> HPKLVSSTPAEGSEGAAPAKIELHFSENLVTQFSGAKLVMTAMPGMEHSPMAVKAAVSGGGDPKTMVITPASPLTAGTYKVDWRAVSSDTFPI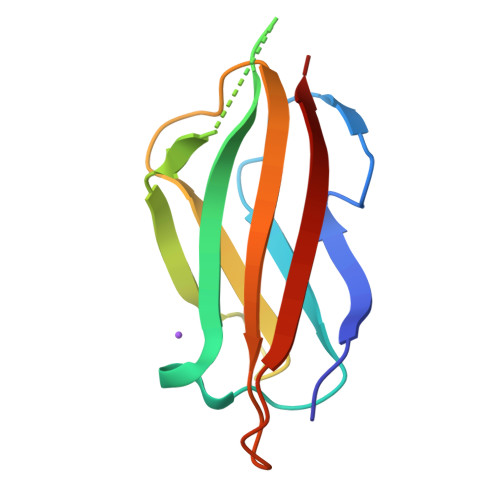TGSVTFKVK> E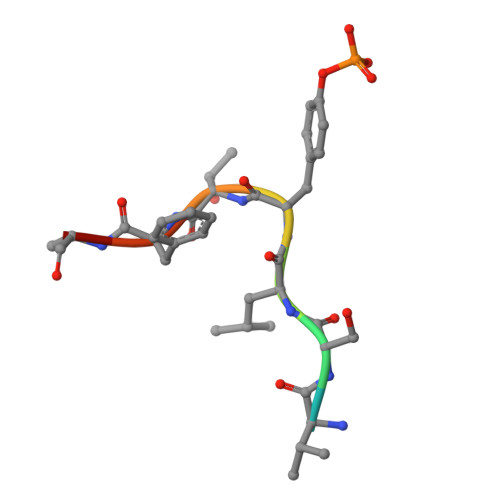VSLYTFDK>[4x]DAKEK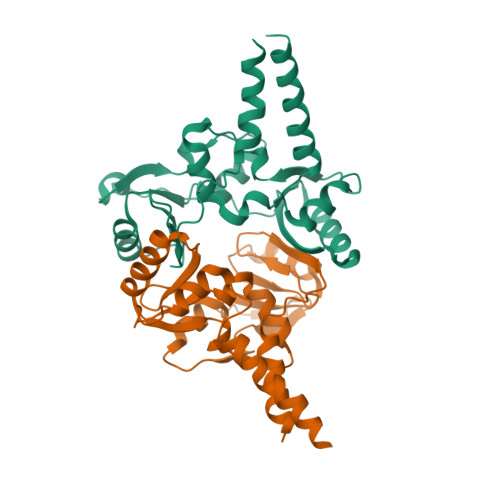RLREIQFEKEMIERDMREYRGFSRAVRAVFEEKERFPGLVDVVSNLIEVDEKYSLAVSVLLGGTAQNIVVRNVDTAKAIVEFLKQNEAGRVTILPLDLIDGSFNRISGLENERGFVGYAVDLVKFPSDLEVLGGFLFGNSVVVETLDDAIRMKKKYRLNTRIATLDGELISGRGAITGGREERSSNVFERRIKLKHLEQEMEETERQI The human proteome comprises 266 human PDZ (PSD95/DLG1/ZO1) domains 16 and about 4000 putative PBMs, defining a network of one million potential interactions. PBMs are mostly (though not exclusively) C-terminal, with their COO- implicated in binding, and are classified based on position −2, being respectively Ser/Thr, hydrophobic or acidic in classes 1, 2, and 3 17,18. PDZ-PBM interactions are rather transient and promiscuous. Viral proteins bearing functional PBMs are found notably in HPV and HTLV oncoviruses as well as in HBV, WNV and coronaviruses including MERS or SARS-CoV213,15,23–26.

The logos of PDZ domains SNTB1 and MAGI1_2 indicate preferences for x-R-E-T-x-V-COO- and R-x-E-T-x-V-COO-, respectively. The oncoviral PBM of HPV35 E6 satisfies both consensus requirements hence recognizes both PDZ domains. The structures of HPV35 E6 PBM bound to both SNTB1 and MAGI1_2 resolve their logo differences by revealing the distinctive contributions of Arg residues at p-4 and p-5 of HPV35 E6 in the two complexes. C MAGI1-2 PDZ logo matches with HPV35 E6 PBM at the same positions, but also at p-5 (Arg), exposed to the acidic β2-β3 loop of MAGI1_2 in the MAGI1/HPV35 E6 complex. Accordingly, HPV35 E6 binds stronger to MAGI1-2 than to SNTB1. Most PBMs in this oncoviral clade share the class 1 consensus E-[TS]-x-V-COO− (where x denotes for any residues), often immediately preceded by basic residue(s). These motifs showed generally high binding affinities with PDZ domains such as MAGI1_2, DLG1_2, SCRIB_1, SNTB1, or TX1BP3.

>[2x]GSMGKPFFTRNPSELKGKFIHTKLRKSSRGFGFTVVGGDEPDEFLQIKSLVLDGPAALDGKMETGDVIVSVNDTCVLGHTHAQVVKIFQSIPIGASVDLELCRGYPLGSSAYGSVKAYTNFDAERDALNIETAIKTKGVDEVTIVNILTNRSNEQRQDIAFAYQRRTKKELASALKSALSGHLETVILGLLKTPAQYDASELKASMKGLGTDEDSLIEIICSRTNQELQEINRVYKEMYKTDLEKDIISDTSGDFRKLMVALAKGRRAEDGSVIDYELIDQDARDLYDAGVKRKGTDVPKWISIMTERSVPHLQKVFDRYKSYSPYDMLESIRKEVKGDLENAFLNLVQCIQNKPLYFADRLYDSMKGKGTRDKVLIRIMVSRSEVDMLKIRSEFKRKYGKSLYYYIQQDTKGDYQKALLYLCGGDD;>TDDSKPTRRETEV[2x]> MSKLASECVANILNDWYIAIKQQDAESAERYFEEVKPLFDEMEEDQEVLMYYSLLEERHKMLLYQVKGEELPPHSYFNENHAEEIKKTDHMIEYYFFLFEALYESHKRNFEKAITLFKIAEKKLKDIPDCIERAEFYSKV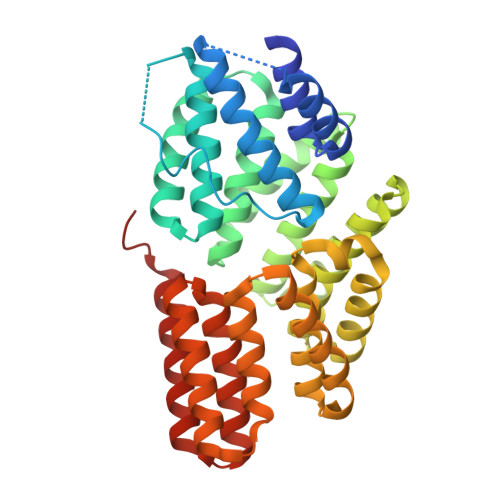ASMYMMLRQSLISLNYINDSIQIYRENEGYKRKLATSLMIVGQNYTDLGLYEKAEESFLEAIRISRVLHDSLFTALIHHNLSITYSAANRSQDCINALKKAIRNKEWRDSVYYINSLYMFLKELYKIGDVNKMPYYYKKTKEYFKRKENKVYEAKINIIYGLLQQDQRKSIETCRGGISYLYEVNDLDSVFDLSLVISEHCEKHGLYKEALEFSKHAILAEEKMRHLEGL> ELCNPQDKQALLQIKKDLGNPTTLSSWLPTTDCCNRTWLGVLCDTDTQTYRVNNLDLSGLNLPKPYPIPSSLANLPYLNFLYIGGINNLVGPIPPAIAKLTQLHYLYITHTNVSGAIPDFLSQIKTLVTLDFSYNALSGTLPPSISSLPNLVGITFDGNRISGAIPDSYGSFSKLFTSMTISRNRLTGKIPPTFANLNLAFVDLSRNMLEGDASVLFGSDKNTQKIHLAKNSLAFDLGKVGLSKNLNGLDLRNNR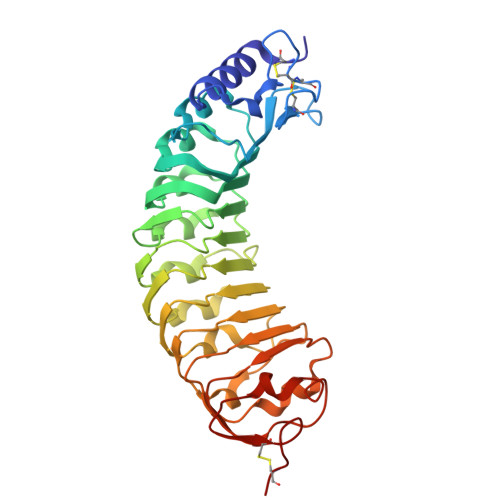IYGTLPQGLTQLKFLHSLDVSFNNLCGEIPQGGNLQRFDVSAYANNKCLCGSPLPACT> XXXXXXXXXXXXXXXXXXXXXXXXXXXXHCAKVLKAIGLQRTGKQEEAFTLAQEVAALEPTDDNSLQALTILYREMHRPELVTKLYEAAVKKVPNSEEYHSHLFMAYARVGEYKKMQQAGMALYKIVPKNPYYFWSVMSLIMQSISAQDENLSKTMFLPLAERMVEKMVKEDKIEAEAEVELYYMILERLGKYQEALDVIRGKLGEKLTSEIQSRENKCMAMYKKLSRWPECNALSRRLLLKNSDDWQFYLTYFDSVFRLIEEAWSPPAEGEHSLEGEVHYSAEKAVKFIEDRITEESKSSRHLRGPHL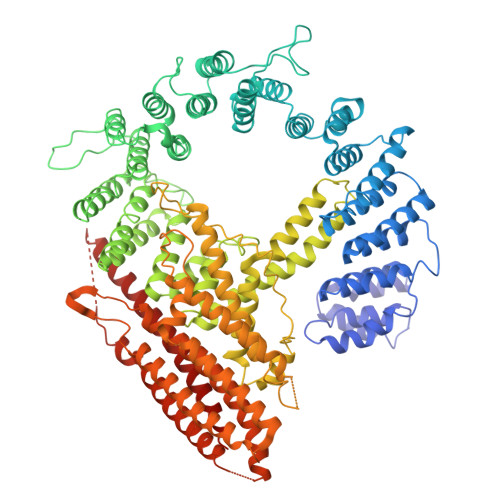AKLELIRRLRSQGCNDEYKLGDPEELMFQYFKKFGDKPCCFTDLKVFVDLLPATQCTKFINQLLGVVPLSTPTEDKLALPADIRALQQHLCVVQLTRLLGLYHTMDKNQKLSVVRELMLRYQHGLEFGKTCLKTELQFSDYYCLLAVHALIDVWRETGDETTVWQALTLLEEGLTHSPSNAQFKLLLVRIYCMLGAFEPVVDLYSSLDAKHIQHDTIGYLLTRYAESLGQYAAASQSCNFALRFFHSNQKDTSEYIIQAYKYGAFEKIPEFIAFRNRLNNSLHFAQVRTERMLLDLLLEANISTSLAESIKSMNLRPEEDDIPWEDLRDNRDLNVFFSWDPKDRDVSEEHKKLSLEEETLWLRIRSLTLRLISGLPSLNHPVEPKNSEKTAENGVSSRIDILRLLLQQLEATLETGKRFIEKDIQYPFLGPVPTRMGGFFNSGCSQCQISSFYLVNDIYELDTSGLEDTMEIQERIENSFKSLLDQLKDVFSKCKGDLLEVKDGNLKTHPTLLENLVFFVETISVILWVSSYCESVLRPYKLNLQKKKKKKKETSIIMPPVFTSFQDYVTGLQTLISNVVDHIKGLETHLIALKLEELILEDTSLSPEERKFSKTVQGKVQSSYLHSLLEMGELLKKRLETTKKLKI>[2x]ANPLYQKHIISINDLSRDDLNLVLATAAKLKANPQPELLKHKVIASCFFE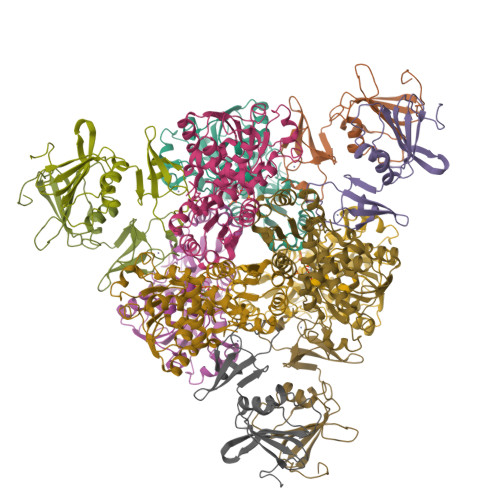ASTRTRLSFETSMHRLGASVVGFSDSANTSLGKKGETLADTISVISTYVDAIVMRHPQEGAARLATEFSGNVPVLNAGDGSNQHPTQTLLDLFTIQQTQGRLDNLHVAMVGDLKYGRTVHSLTQALAKFDGNRFYFIAPDALAMPEYILDMLDEKGIAWSLHSSIEEVMAEVDILYMTRVQKERLDPSEYANVKAQFVLRASDLHNAKANMKVLHPLPRVDEIATDVDKTPHAWYFQQAGNGIFARQALLALVLNRDLVL;>[2x]MTHDNKLQVEAIKRGTVIDHIPAQIGFKLLSLFKLTETDQRITIGLNLPSGEMGRKDLIKIENTFLSEDQVDQLALYAPQATVNRIDNYEVVGKSRPSLPERIDNVLVCPNSNCISHAEPVSSSFAVRKRANDIALKCKYCEKEFSHNVVLAN>MLTEEFVSAICGPPLSSNTAIAKDVGIYCHTLSPSYSVKSTFKKSSVPVNCLAVSDTHIFAGQHEKAYVHVYSRLRGNQEAFVALPERIRCLILIGDILVVGTTEGRLMLWEICTGRLVSTPARHVQAVSCVAATPSHVLTGSDDSDIHVWSLSQLLELDSAAEHEPLRTLANHRAAITALAVSPSDSADTNFCVSASKDKSCIIWNYQTGDALRTLIFPGYPLCMSLDPSSRAIFVSCEDSSLYVAEMFGEKPLLGPGSEDPSTVVQISTPFGATQPDVGPASCLSVSYDGTMLLTGHPRGQIMRWDISENKSPVELANLNAAVTNLIFVSPFLTSKPTKTVNIIKPSQAERAYTFTAQFEPMSFTKSRLDSLLNATGFPADALESAIVAFYQPVTQSAGDQELQRQNEELWEIINEQRALQKETLQRYVEAKSSR[2x];>MTAPPDLRVVCHRLASTPVDSLPRLCPLLINHVLRCGGPLSEPQDAKGKDRTSETAMLVHKFRTHITSLLTGKSPAGRFTAVCLIKAVIDVGGWESLRSAEPWIRGLIGVLQKPDPLSSKELSIVTLTKLYILLQDYQTLIREMATPTLPGYATACLQLIKPPASGRPLKVPLNFVDTVAWSLSKLVVLYSTTMRPFSGQIKSALRPYIAPTSSDNVVVPQSLKENSRNLLILLTYTAPKNGSSDEWVKAIRATILDCHTTADQVFRAVRESWESTTGYHIQPVNATGEPSGGGDSVDELPPWSGLQAGAERLTGLLEYLTAYFNNPTRAPVNVPLGELLDLTTRLTLVIPPSLGAEDSIETNPAIGRDEKAELWSALPDIHHAVLRLHCAIIRRLEANAIPLATDIIDQMVRVSTASKQLPSVRETAYILA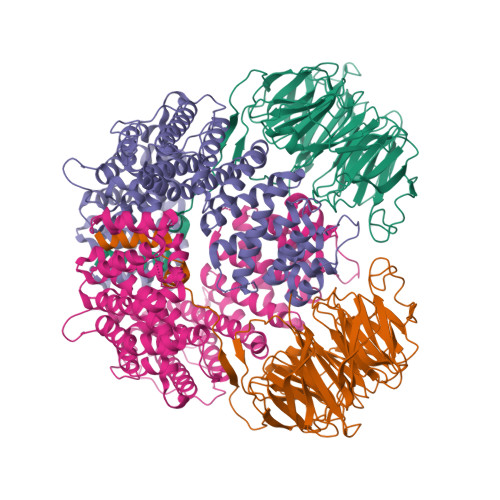KEILLLAGSTLPKLTVDILIPLIQSSCHDILTAAGHAQPAQSQSSVPVTASKQQKSSSPALTNADAFLPGQSSSSTPKTSTASPVSQAASALLPTFFTHLPQKHLPPDIRGLLDRTAILSHNQSAMLASCLHPYRDSRGRYYPSILPFLVRRFPRDESVEVLRSNLVKVGGSDASRGWDLSNGVTRDISYGREFAQEMISEEKGVVKEDETFAKEIEPVKSTAKPATSANAWGVEMELDVEHVNVAPIPETTNPFATVVGTTSQPSTLIQPACPSSPLKRKSDAEEFDEGSRPKRVDTGKAVSHPQMAVISSVPKPEEDKSDESSDSEGSVQIDMTLEDDEEDEEEEDE[2x]> ASITDKDHQKVILVGDGAVGSSYAFAMVLQGIAQEIGIVDIFKDKTKGDAIDLSNALPFTSPKKIYSAEYSDAKDADLVVITAGAPKQPGETRLDLVNKNLKILKSIVDPIVDSGFN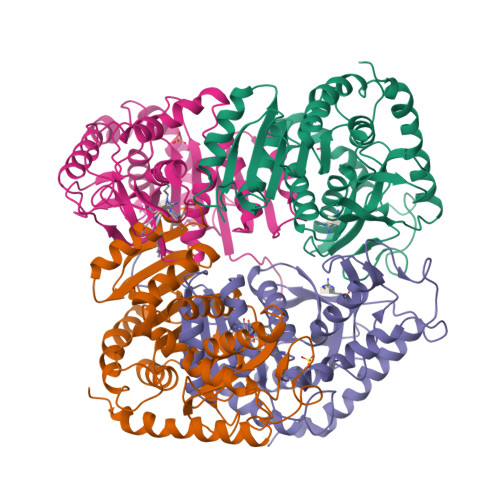LIFLVAANPVDILTYATWKLSGFPKNRVVGSGTSLDTARFRQSIAEMVNVDARSVHAYIMGEHGDTEFPVWSHANIGGVTIAEWVKAHPEIKEDKLVKMFEDVRDAAYEIIKLKGATFYGIATALARISKAILNDENAVLPLSVYMDGQYGINDLYIGTPAVINRNGIQNILEIPLTDHEEESMQKSASQLKKVLTDAFAKNDIETRQ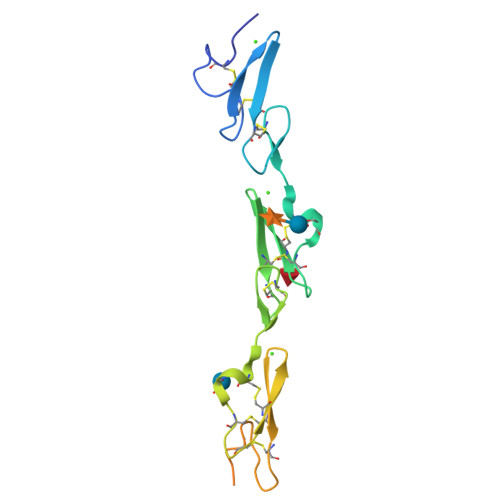> EDVDECAMANSNPCEHAGKCVNTDGAFHCECLKGYAGPRCEMDINECHSDPCQNDATCLDKIGGFTCLCMPGFKGVHCELEINECQSNPCVNNGQCVDKVNRFQCLCPPGFTGPVCQIDGSGLEVLFQGPGSLHHILDAQKMVWNHRGHHHHHHHH4-{2-[(cyclopropylmethyl)amino]-5-(ethylsulfonyl)phenyl}-6-methyl-1,6-dihydro-7H-pyrrolo[2,3-c]pyridin-7-one | C20 H23 N3 O3 S | 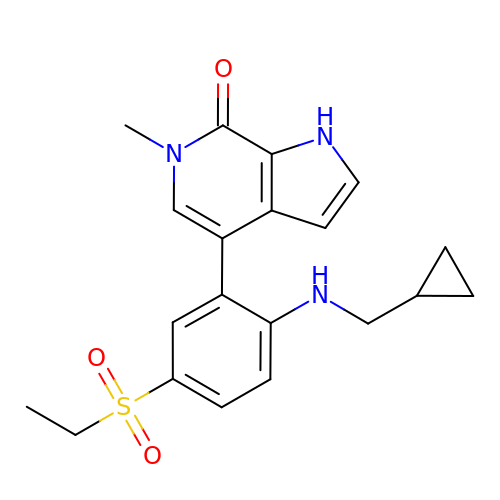ZQRYCQNBELIIBM-UHFFFAOYSA-N>[2x]SMAKIIFPEDFIWGAATSSYQIEGAFNEDGKGESIWDRFSHTPGKIENGDTGDIACDHYHLYREDIELMKEIGIRSYRFSTSWPRILPEGKGRVNQKGLDFYKRLVDNLLKANIRPMITLYHWDLPQALQDKGGWTNRDTAKYFAEYARLMFEEFNGLVDLWVTHNEPWVVAFEGHAFGNHAPGTKDFKTALQVAHHLLLSHGMAVDIFREEDLPGEIGITLNLTPAYPAGDSEKDVKAASLLDDYINAWFLSPVFKGSYPEELHHIYEQNLGAFTTQPGDMDIISRDIDFLGINYYSRMVVRHKPGDNLFNAEVVKMEDRPSTEMGWEIYPQGLYDILVRVNKEYTDKPLYITENGAAFDDKLTEEGKIHDEKRINYLGDHFKQAYKALKDGVPLRGYYVWSLMDNFEWAYGYSKRFGLIYVDYENGNRRFLKDSALWYREVIEKGQVEAN

In this work, a BGL from the thermophilic and halophilic bacterium Halothermothrix orenii, HoBGLA, was characterized biochemically and structurally. It is an unspecific β-glucosidase with mixed activities for different substrates and prominent activity with various galactosidases such as lactose. The overall structure of the 451-residue large HoBGLA displays the typical (β/α)8 TIM-barrel fold adopted by retaining GH1 enzymes. In subsite −1 of the active site, the catalytic residues Glu354 (nucleophile) and Glu166 (acid/base catalyst) are situated near Glu408.

The crystal structure of HoBGLA in complex with thiocellobiose, HoBGLA–TCB, was determined at 1.85 Å resolution, and shows well-defined electron density for the TCB ligand. In HoBGLA, however, the TCB molecules folds into an unusual conformation to place the reducing end O1 atom within short hydrogen-bonding distance of the catalytic nucleophile Glu354 Oε2 atom. Considering the overall similarity of the active site in HoBGLA and PpBGLB, the striking difference in TCB binding was unexpected. The corresponding loop in HoBGLA is considerably shorter (residues 303–308), which provides more space in this region of the cleft. Consequently, the PEG molecule is allowed to bind differently in +4 than the corresponding glucosyl unit in cellopentaose bound to BGlu1. We predict that an oligosaccharide longer than four sugar units, i.e., binding beyond subsite +3, could be bound to HoBGLA either as observed for the cellopentaose in BGlu1, or possibly, as observed for PEG in the TCB complex.>MGYLNREERRETIMQAAMRVALDQGFTGMTVRNIATAAGVAAGQVHHHFTSSGELKSQAFIRVIREMMDLQRLSRTAGWREQLFSALGSEDGRLEPYIRLWRQAQLLADSDPEIKSAYLLTMNLWHDEAVRIIRAGHAAGEFTLRDSAENIAWRLIS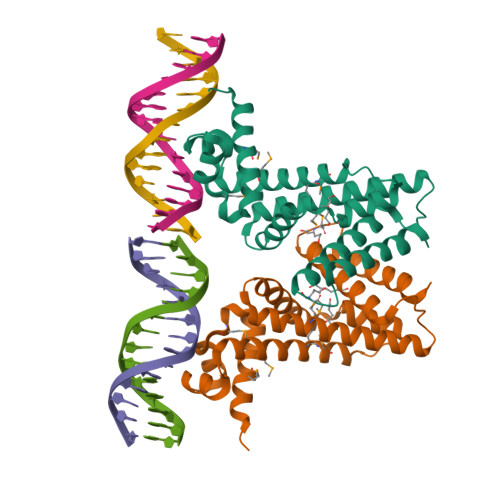LVCGLDGIYVLGMPEVDDAAFTRHLQHVIQLELFS[4x]> XXXXXXXXXXXXXXXXXXXXXXXXXXXXXXXXXXXXXXXXXXXXXXXXXXXXXXXXXXXXXXXXXXXXXXXXXXXXXXXXXXXXXXXXXX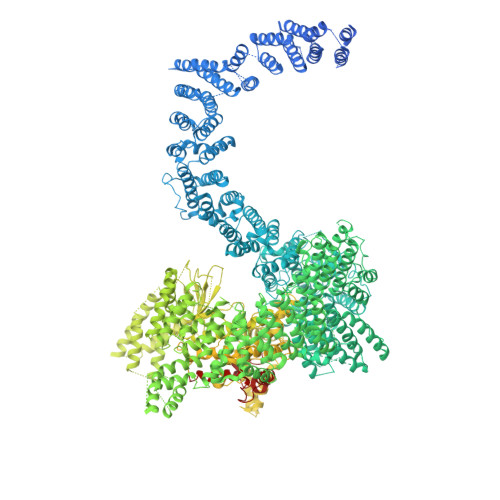XXXXXXXXXXXXXXXXXXXXXXXXXXXXXXXXXXXXXXXXXXXXXXXXXXXXXXXXXXXXXXXXXXXXXXXXXXXXXXXXXXXXXXXXXXXXXXXXXXXXXXXXXXXXXXXXXXXXXXXXXXXXXXXXXXXXXXXXXXXXXXXXXXXXXXXXXXXXXXXXXXXXXXXXXXXXXXXXXXXXXXXXXXXXXXXXXXXXXXXXXXXXXXXXXXXXXXXXXXXXXXXXXXXXXXXXXXXXXXXXXXXXXXXXXXXXXXXXXXXXXXXXXXXXXXXXFSTNFRDTVDILVGWHIDHTQKPSLTQQVSGWLQSLEPFWVADLAFSTTLLGQFLEDMEAYAEDLSHVASGESVDEDVPPPSVSLPKLAALLRVFSTVVRSIGERFSPIRGPPITEAYVTDVLYRVMRCVTAANQVFFSEAVLTAANECVGVLLGSLDPSMTIHCDMVITYGLDQLENCQTCGTDYIISVLNLLTLIVEQINTKLPSSFVEKLFIPSSKLLFLRYHKEKEVVAVAHAVYQAVLSLKNIPVLETAYKLILGEMTCALNNLLHSLQLPEACSEIKHEAFKNHVFNVDNAKFVVIFDLSALTTIGNAKNSLIGMWALSPTVFALLSKNLMIVHSDLAVHFPAIQYAVLYTLYSHCTRHDHFISSSLSSSSPSLFDGAVISTVTTATKKHFSIILNLLGILLKKDNLNQDTRKLLMTWALEAAVLMRKSETYAPLFSLPSFHKFCKGLLANTLVEDVNICLQACSSLHALSSSLPDDLLQRCVDVCRVQLVHSGTRIRQAFGKLLKSIPLDVVLSNNNHTEIQEISLALRSHMSKAPSNTFHPQDFSDVISFILYGNSHRTGKDNWLERLFYSCQRLDKRDQSTIPRNLLKTDAVLWQWAIWEAAQFTVLSKLRTPLGRAQDTFQTIEGIIRSLAAHTLNPDQDVSQWTTADNDEGHGNNQLRLVLLLQYLENLEKLMYNAYEGCANALTSPPKVIRTFFYTNRQTCQDWLTRIRLSIMRVGLLAGQPAVTVRHGFDLLTEMKTTSLSQGNELEVTIMMVVEALCELHCPEAIQGIAVWSSSIVGKNLLWINSVAQQAEGRFEKASVEYQEHLCAMTGVDCCISSFDKSVLTLANAGRNSASPKHSLNGESRKTVLSKPTDSSPEVINYLGNKACECYISIADWAAVQEWQNAIHDLKKSTSSTSLNLKADFNYIKSLSSFESGKFVECTEQLELLPGENINLLAGGSKEKIDMKKLLPNMLSPDPRELQKSIEVQLLRSSVCLATALNPIEQDQKWQSITENVVKYLKQTSRIAIGPLRLSTLTVSQSLPVLSTLQLYCSSALENTVSNRLSTEDCLIPLFSEALRSCKQHDVRPWMQALRYTMYQNQLLEKIKEQTVPIRSHLMELGLTAAKFARKRGNVSLATRLLAQCSEVQLGKTTTAQDLVQHFKKLSTQGQVDEKWGPELDIEKTKLLYTAGQSTHAMEMLSSCAISFCKSVKAEYAVAKSILTLAKWIQAEWKEISGQLKQVYRAQHQQNFTGLSTLSKNILTLIELPSVNTMEEEYPRIESESTVHIGVGEPDFILGQLYHLSSVQAPEVAKSWAALASWAYRWGRKVVDNASXXXXXXXXXXXXXXXXXXXXXXXXXXXXXXXXXXXXXXXXXXXXXXXXXXXXXXXXXXXXXXXXXXXXXXXXXXXXXXXXXXXXXXXXEGVIKVWRKVVDRIFSLYKLSCSAYFTFLKLNAGQIPLDEDDPRLHLSHRVEQSTDDMIVMATLRLLRLLVKHAGELRQYLEHGLETTPTAPWRGIIPQLFSRLNHPEVYVRQSICNLLCRVAQDSPHLILYPAIVGTISLSSESQASGNKFSTAIPTLLGNIQGEELLVSECEGGSPPASQDSNKDEPKSGLNEDQAMMQDCYSKIVDKLSSANPTMVLQVQMLVAELRRVTVLWDELWLGVLLQQHMYVLRRIQQLEDEVXXXXXXXXXXXXXXXXXXXXXXXXXXXXXXXXXXXXXXXXXXXXXXPHEKWFQDNYGDAIENALEKLKXXXXXXXXXXXXXXXXXXXXXXXXXXXXXXYILRLEEISPWLAAMTNTEIALPGEVSARDTVTIHSVGGTITILPTKTKPKKLLFLGSDGKSYPYLFKGLEDLHLDERIMQFLSIVNTMFATINRQETPRFHARHYSVTPLGTRSGLIQWVDGATPLFGLYKRWQQREAALQAQKXXXXXXXXXXXXXXXXXXXXXXXXXXXXXXXXXXXXXXXXXXWPLHVMKAVLEELMEATPPNLLAKELWSSCTTPDEWWRVTQSYARSTAVMSMVGYIIGLGARHLDNVLIDMTTGEVVHIDYNVCFEKGKSLRVPEKVPFRMTQNIETALGVTGVEGVFRLSCEQVLHIMRRGRETLLTLLEAFVYDPLVDWTAGGEAGFAGAVYGGGGQQAESKQSKREMEREITRSLFSSRVAEIKVNWFKNRDEMLVVLPKLDGSLDEYLSLQEQLTDVEKLQGKLLEEIEFLEGAEGVDHPSHTLQHRYSEHTQLQTQQRAVQEAIQVKLNEFEQWITHYQAAFNNLEATQLASLLQEISTQMDLGPPSYVPATAFLQNAGQAHLISQCEQLEGEVGALLQQRRSVLRGCLEQLHHYATVALQYPKAIFQKHRIEQWKTWMEELICNTTVERCQELYRKYEMQYAPQPPPTVCQFITATEMTLQRYAADINSRLIRQVERLKQEAVTVPVCEDQLKEIERCIKVFLHENGEEGSLSLASVIISALCTLTRRNLMMEGAASSAGEQLVDLTSRDGAWFLEELCSMSGNVTCLVQLLKQCHLVPQDLDIPNPMEASETVHLANGVYTSLQELNSNFRQIIFPEALRCLMKGEYTLESMLHELDGLIEQTTDGVPLQTLVESLQAYLRNAAMGLEEETHAHYIDVARLLHAQYGELIQPRNGSVDETPKMSAGQMLLVAFDGMFAQVETAFSLLVEKLNKMEIPIAWRKIDIIREARSTQVNFFDDDNHRQVLEEIFFLKRLQTIKEFFRLCGTFSKTLSGSSSLEDQNTVNGPVQIVNVKTLFRNSCFSEDQMAKPIKAFTADFVRQLLIGLPNQALGLTLCSFISALGVDIIAQVEAKDFGAESKVSVDDLCKKAVEHNIQIGKFSQLVMNRATVLASSYDTAWKKHDLVRRLETSISSCKTSLQRVQLHIAMFQWQHEDLLINRPQAMSVTPPPRSAILTSMKKKLHTLSQIETSIATVQEKLAALESSIEQRLKWAGGANPALAPVLQDFEATIAERRNLVLKESQRASQVTFLCSNIIHFESLRTRTAEALNLDAALFELIKRCQQMCSFASQFNSSVSELELRLLQRVDTGLEHPIGSSEWLLSAHKQLTQDMSTQRAIQTEKEQQIETVCETIQNLVDNIKTVLTGHNRQLGDVKHLLKAMAKDEEAALADGEDVPYENSVRQFLGEYKSWQDNIQTVLFTLVQAMGQVRSQEHVEMLQEITPTLKELKTQSQSIYNNLVSFASPLVTDATNECSSPTSSATYQPSFAAAVRSNTGQKTQPDVMSQNARKLIQKNLATSADTPPSTVPGTGKSVACSPKKAVRDPKTGKAVQERNSYAVSVWKRVKAKLEGRDVDPNRRMSVAEQVDYVIKEATNLDNLAQLYEGWTAWV> MRGSHHHHHHGIPEFVNALVSHLLVVEPEKLYAM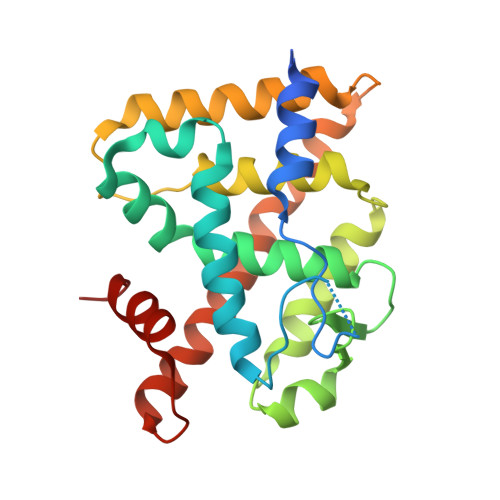PDPAGPDGHLPAVATLCDLFDREIVVTISWAKSIPGFSSLSLSDQMSVLQSVWMEVLVLGVAQRSLPLQDELAFAEDLVLDEEGARAAGLGELGAALLQLVRRLQALRLEREEYVLLKALALANSDSVHIEDAEAVEQLREALHEALLEYEAGRAGPGGGAERRRAGRLLLTLPLLRQTAGKVLAHFYGVKLEGKVPMHKLFLEMLEAMMD> ACTKNAIAQTGFNKDKYFNGDVWYVTDYLALEPDDVPKRYCAA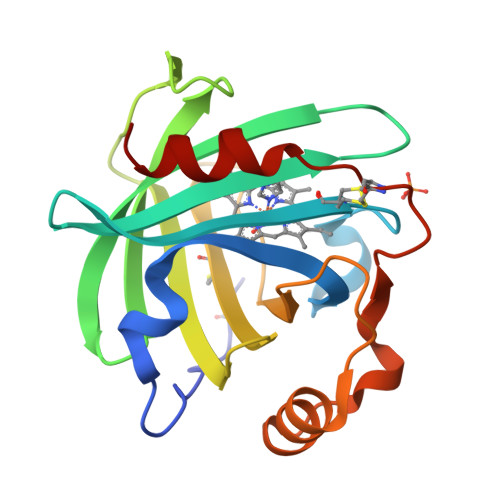LAAGTASGKLKEALYHYDPKTQDTFYDVSELQVESLGKYTANFKKVDKNGNVKVAVTAGNYYTFTVMYADDSSALIHTCLHKGNKDLGDLYAVLNRNKDAAAGDKVKSAVSAATLEFSKFISTKENNCAYDNDSLKSLLTK> MAYKRSQILICGGTGCTSSGSMVLVKELKKELVKHDILDEVEVVTTGCFGLCELGPVVIVYPEGTFYSRVEAADIPEMVEEHLVKGRPLDRLIYNEKGDGHHPLSINELGFFKKQRRIALANCGVINPENIDEYIGFDGYLALEKVLLTMSPVDVINEVKASGLRGRGGGGFPTGLKWQFAHDAVSEDGIKYVACNADEGDPGAFMDRSVLEGDPHAVIEAMAIAGYAVGASKGYVYVRAEYPIAVNRLQIAIDQAKEYGILGENIFETDFSFDLEIRLGAGAFVCGEETALMNSIEGKRGEPRPRPPFPANKGLFGKPTVLNNVETYANIPKIILNGAEWFASVGTEKSKGTKVFALGGKINNTGLLEIPMGTTLREIIYEIGGGIPNGKAFKAAQTGGPSGGCLPESLLDTEIDYDNLIAAGSMMGSGGLIVMDEDNCMVDVARFFLDFTQDESCGKCPPCRIGTKRMLEILERICDGKGVEGDIERLEELAVGIKSSALCGLGQTAPNPVLSTIRFFRDEYEAHIRDKKCPAGVCKHLLDFKINADTCKGCGICAKKCPADAISGEKKKPYNIDTSKCIKCGACIEAC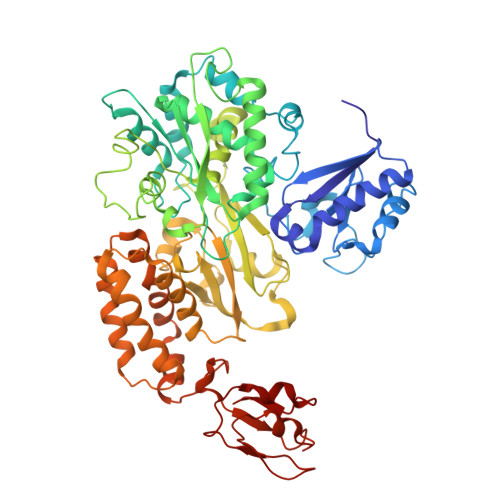PFGSISKA>[3x]MTSFTIPGLSDKKASDVADLLQKQLSTYNDLHLTLKHVHWNVVGPNFIGVHEMIDPQVELVRGYADEVAERIATLGKSPKGTPGAIIKDRTWDDYSVERDTVQAHLAALDLVYNGVIE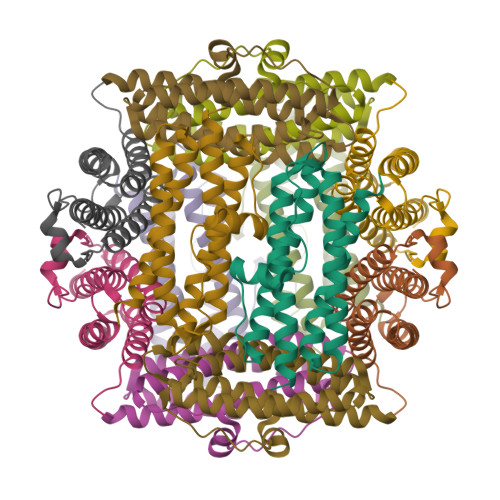DTRKSIEKLEDLDLVSQDLLIAHAGELEKFQWFVRAHLESAGGQLTHEGQSTEKGAADKARRKSA> MSQRITIDPVTRIEGHLRIDCEIENGVVSKAWASGTMWRGMEEIVKNRDPRDAWMIVQRICGVCTTTHALSSVRAAESA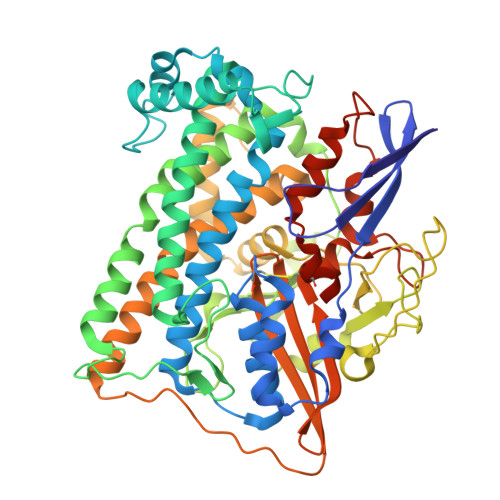LNIDVPVNAQYIRNIILAAHTTHDHIVHFYQLSALDWVDITSALQADPTKASEMLKGVSTWHLNSPEEFTKVQNKIKDLVASGQLGIFANGYWGHPAMKLPPEVNLIAVAHYLQALECQRDANRVVALLGGKTPHIQNLAVGGVANPINLDGLGVLNLERLMYIKSFIDKLSDFVEQVYKVDTAVIAAFYPEWLTRGKGAVNYLSVPEFPTDSKNGSFLFPGGYIENADLSSYRPITSHSDEYLIKGIQESAKHSWYKDEAPQAPWEGTTIPAYDGWSDDGKYSWVKSPTFYGKTVEVGPLANMLVKLAAGRESTQNKLNEIVAIYQKLTGNTLEVAQLHSTLGRIIGRTVHCCELQDILQNQYSALITNIGKGDHTTFVKPNIPATGEFKGVGFLEAPKGMLSHWMVIKDGIISNYQAVVPSTWNSGPRNFNDDVGPYEQSLVGTPVADPNKPLEVVRTIHSFDPCMACAVHVVDADGNEVVSVKVL> AKEMKPFPQQVNYAGVIKPNHVTQESLNASV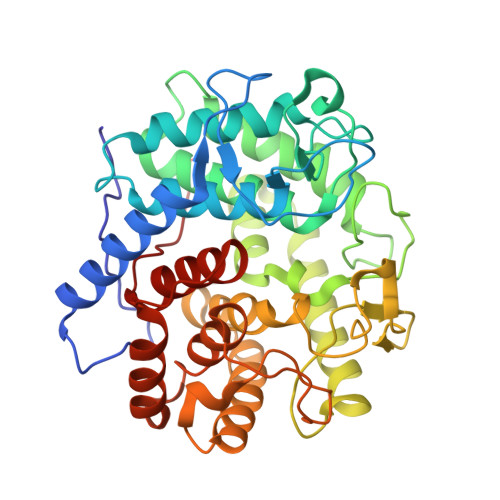RSYYDNWKKKYLKNDLSSLPGGYYVKGEITGDADGFKPLGTSEGQGYGMIITVLMAGYDSNAQKIYDGLFKTARTFKSSQNPNLMGWVVADSKKAQGHFDSATDGDLDIAYSLLLAHKQWGSNGTVNYLKEAQDMITKGIKASNVTNNNQLNLGDWDSKSSLDTRPSDWMMSHLRAFYEFTGDKTWLTVINNLYDVYTQFSNKYSPNTGLISDFVVKNPPQPAPKDFLDESEYTNAYYYNASRVPLRIVMDYAMYGEKRSKVISDKVSSWIQNKTNGNPSKIVDGYQLNGSNIGSYPTAVFVSPFIAASITSSNNQKWVNSGWDWMKNKRERYFSDSYNLLTMLFITGNWWKPVP1-~{tert}-butyl-~{N}-[(5~{R})-8-[2-[(1-methylpyrazol-4-yl)amino]pyrimidin-4-yl]-2-(oxetan-3-yl)-1,3,4,5-tetrahydro-2-benzazepin-5-yl]-1,2,3-triazole-4-carboxamide | C28 H34 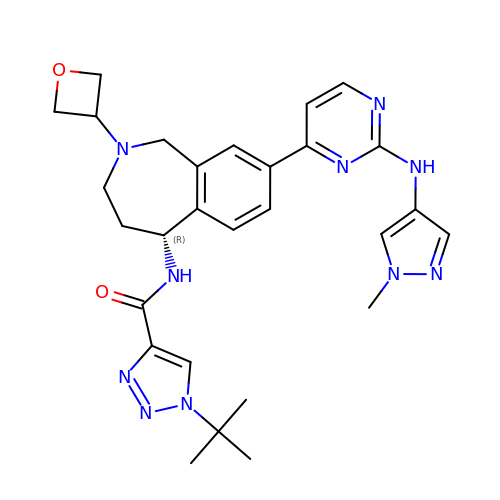N10 O2 | JSAQBOQCZJHWMA-XMMPIXPASA-N5-(3,7,11,15,19,23-HEXAMETHYL-TETRACOSA-2,6,10,14,18,22-HEXAENYL)-2,3-DIMETHOXY-6-METHYL-BENZENE-1,4-DIOL | C39 H60 O4 | 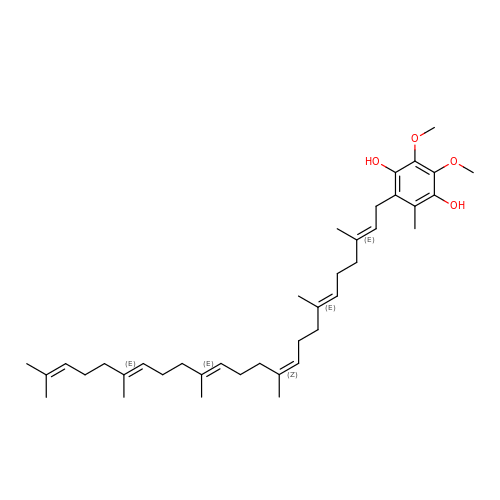DYOSCPIQEYRQEO-XQCASOQKSA-N>SPLAAYEVDDSTGYLTSDVGGPIQDQTSLKAGIRGPTLLEDFMFRQKIQHFDHERVPERAVHARGAGAHGTFTSYADWSNITAASFLNATGKQTPVFVRFSTVAGSRGSADTARDVHGFATRFYTDEGNFDIVGNNIPVFFIQDAIQFPDLIHSVKPRPDNEIPQAATAHDSAWDFFSQQPSTMHTLFWAMSGHGIPRSYRHMDGFGVHTFRFVKDDGSSKLIKWHFKSRQGKASLVWEEAQVLSGKNADFHRQDLWDAIESGNGPEWDVCVQIVDESQAQAFGFDLLDPTKIIPEEYAPLTKLGLLKLDRNPTNYFAETEQVMFQPGHIVRGIDFTEDPLLQGRLFSYLDTQLNRNGGPNFEQLPINMPRVPIHNNNRDGAGQMFIHRNKYPYTPNTLNSGYPRQANQNAGRGFFTAPGRTASGALVREVSPTFNDHWSQPRLFFNSLTPVEQQFLVNAMRFEISLVKSEEVKKNVLTQLNRVSHDVAVRVAAAIGLGAPDADDTYYHNNKTAGWSIVGSGPLPTIKTLRVGILATTSESS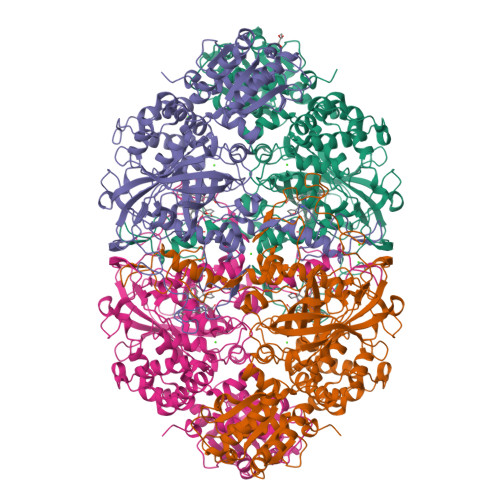ALDQAAQLRTRLEKDGLVVTVVAETLREGVDQTYSTADATGFDGVVVVDGAAALFASTASSPLFPTGRPLQIFVDAYRWGKPVGVCGGKSSEVLDAADVPEDGDGVYSEESVDMFVEEFEKGLATFRFTDRFALDS[4x]N~3~,N~3~-bis[(2H-1,3-benzodioxol-5-yl)methyl]-N-hydroxy-beta-alaninamide 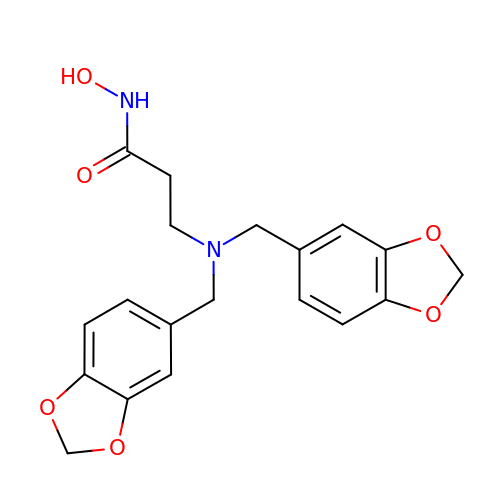| C19 H20 N2 O6 | BSWWAZYKBXDQTA-UHFFFAOYSA-N> GMREEKIREALNAHWQASAAGDFDAEHDIYDDDAICDYPQSGERILGRMNLQALRSHHPGKPAGF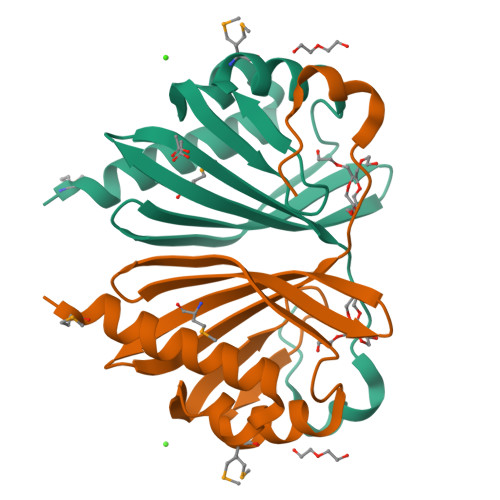EVRRIQGEGNLWITEYSISYNGRPAYTVSIMEFRNGKVVHETQYFSDPFEAPGWRSQWVQQIG>MRDTDVTVLGLGLMGQALAGAFLKDGHATTVWNRSEGKAGQLAEQGAVLASSARDAAEASPLVVVCVSDHAAVRAVLDPLGDVLAGRVLVNLTSGTSEQARATAEWAAERGITYLDGAIMAIPQVVGTADAFLLYSGPEAAYEAHEPTLRSLGAGTTYLGADHGLSSLYDVALLGIMWGTLNSFLHGAALLGTAKVEATTF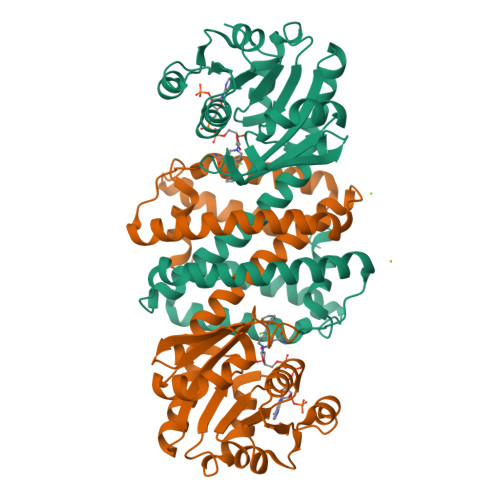APFANRWIEAVTGFVSAYAGQVDQGAYPALDATIDTHVATVDHLIHESEAAGVNTELPRLVRTLADRALAGGQGGLGYAAMIEQFRSPSA[6x]> MRSCRRSVAQHPCAIQVDIVAMAAFISSFAGAQLAHARPSKQTALRAALTLPGTAETNLAVPSNAVRKVQPYPIAKPPSYSSVDSLRPARVSRMDADWATIYEQVRRQVMGNAYVMEGEAPDIDVAFSQLKGGNLTVREFVRAVGKSASYRTRFMEAKSSYNFVLLNFKHFLGRAPTQEEVSTHIQILATSGLEAEID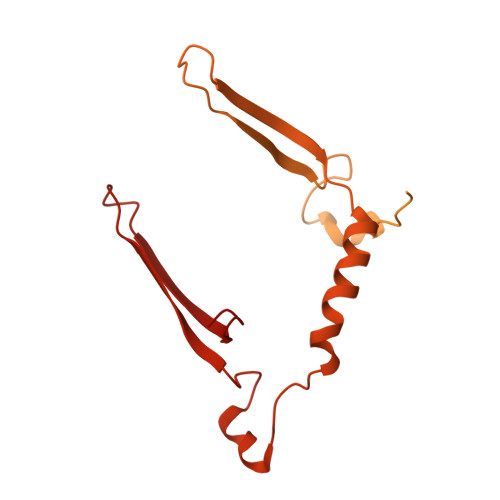SYIDSDEYKALFGDHVVPYVVYRGTYLSSERFNRMVKANPGGATSDKAKSNLNMIATVAADLPTDAIDVMRGLPSPITSETLAFGTAYYWAKVEKEASEGRSASPIGEKIGKFDHAPISTYTSLCSYDKVNKAPQISVTNVGSDEHSYVSVTSKYIAPDMAAAAQMLADCQKYKAGGNAPTGKWMKYYPGTTVNMAPYISLNDTGSDSSRTVSVTLDKVKISPNKIGK> GPGHERREVPNASGSAILNVAKSRIGKQYMSGGTGPDLFDCSGLVLYSHNQCGVYGVPRVAKDQARGGKAGSGAAGDVVYFGNPAHHVGICCGDGSMVHAPRPGKTVCILKIAYMKES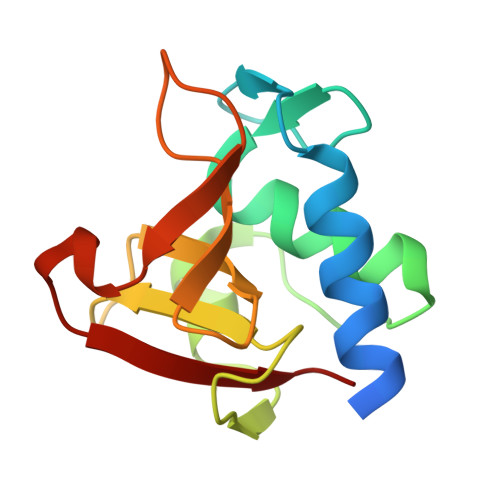YGYRRYY> NPIHDRTSDYHKYLKVKQGDSDLFKLTVSDKRYIWYNPDPKERDSYECGEIVSETSDSFTFKTVDGQDRQVKKDDANQRNPIKFDGVEDMSELSYLNEPAVFHNLRVRYNQDLIYTYSGLFLVAVNPFKRIPIYTQEMVDIFKGRRRNEVAPHIFAISDVAYRSMLDDRQNQSLLITGESGAGKTENTKKVIQYLASVAGRNQANGSGVLEQQILQANPILEAFGNAKTTRNNNSSRFGKFIEIQFNSAGFISGASIQSYLLEKSRVVFQSETERNYHIFYQLLAGATAEEKKALHLAGPESFNYLNQSGCVDIKGVSDSEEFKITRQAMDIVGFSQEEQMSIFKIIAGILHLGNIKFEKGAGEGAVLKDKTALNAASTVFGVNPSVLEKALMEPRILAGRDLVAQHLNVEKSSSSRDALVKALYGRLFLWLVKKINNVLCQERKAYFIGVLDISGFEIFKVNSFEQLCINYTNEKLQQFFNHHMFKLEQEEYLKEKINWTFIDFGLDSQATIDLIDGRQPPGILALLDEQSVFPNATDNTLITKLHSHFSKKNAKYEEPRFSKTEFGVTHYAGQVMYEIQDWLEKNKDPLQQDLELCFKDSSDNVVTKLFNDPNIASRAKKGANFITVAAQYKEQLASLMATLETTNPHFVRCIIPNNKQLPAKLEDKVVLDQLRCNGVLEGIRITRKGFPNRIIYADFVKRYYLLAPNVPRDAEDSQKATDAVLKHLNIDPEQYRFGITKIFFRAGQLARIEEAREQRLESNEPP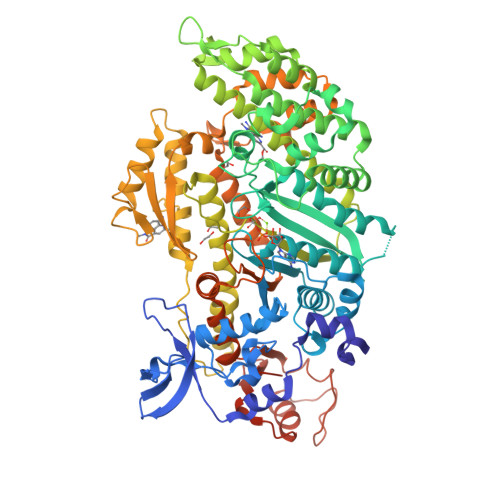MDFDDDIPF> GSHMDSTTIQQNKDTLSQIVVFPTGNYDKNEANAMVNRLANIDGKYLNALKQNNLKIKLLSGKLTDEKEYAYLKGVVPKGWEGTGKTWDDVPGLGGSTVALRIGFSNKGKGHDAINLELHATAHAIDHIVLN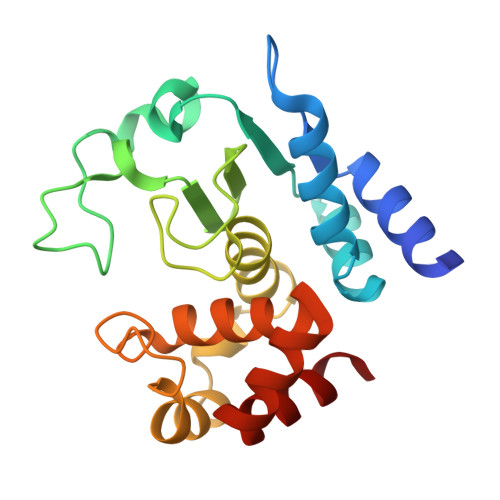DISKSAQFKQIFAKEGRSLGNVNFLGVYPEEFFAESFAYYYLNQDTNSKLKSACPQTYSFLQNLAK> GTSTQTKAGSLTIVGTGIESIGQMTLQALSYIEAAAKVFYCVIDPATEAFILTKNKNCVDLYQYYDNGKSRLNTYTQMSELMVREVRKGLDVVGVFYGHPGVFVNP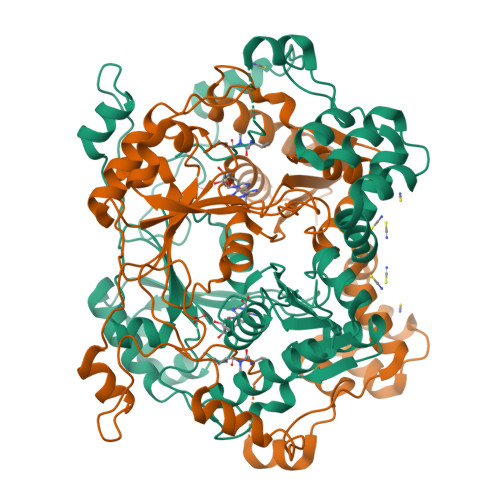SHRALAIAKSEGYRARMLPGVSAEDCLFADLCIDPSNPGCLTYEASDFLIRDRPVSIHSHLVLFQVGCVGIADFNFTGFDNNKFGVLVDRLEQEYGAEHPVVHYIAAMMPHQDPVTDKYTVAQLREPEIAKRVGGVSTFYIPPKARKASNLDIIRRLELLPAGQVPDKKARIYPANQWEPDVPEVEPYRPSDQAAIAQLADHAPPEQYQPLATSKAMSDVMTKLALDPKALADYKADHRAFAQSVPDLTPQERAALELGDSWAIRCAMKNMPSSLLDAARESGEEASQNGFPAVIVVGVIGVIG> PISPIETVPVKLKPGMDGPKVKQWPLTEEKIKALVEICTEMEKEGKISKIGPENPYNTPVFAIKKKDSTKWRKLVDFRELNKRTQDFWEVQLGIPHPAGIKKKKSVTVLDVGDAYFSVPLDEDFRKYTAFTIPSINNETPGIRYQYNVLPQGWKGSPAIFQSSMTKILEPFRKQNPDIVIYQYMDDLYVGSDLEIGQHRTKIEELRQHLLRWGLTTPDKKHQKEPPFLWMGYELHPDKWTVQPIVLPEKDSWTVNDIQKLVGKLNWASQIYPGIKVRQLCKLLRGTKALTEVIPLTEEAELELAENREILKEPVHGVYYDPSKDLIAEIQKQGQGQWTYQIYQEPFKNLKTGKYARMRGAHTNDVKQLTEAVQKITTESIVIWGKTPKFKLPIQKETWETWWTEYWQATWIPEWEFVNTPPLVKLWYQLEKEPIVGAETFYVDGAANRETKLGKAGYVTNRGRQKVVTLTDTTNQKTELQAIYLALQDSGLEVNIVTDSQYALGIIQAQPDQSESELVNQIIEQLIKKEKVYLAWVPAHKGIGGNEQVDKLVSAGIRKVL;> PISPIETVPVKLKPGMDGPKVKQWPLTEEKIKALVEICTEMEKEGKISKIGPENPYNTPVFAIKKKDSTKWRKLVDFRELNKRTQDFWEVQLGIPHPAGIKKKKSVTVLDVGDAYFSVPLDEDFRKYTAFTIPSINNETPGIRYQYNVLPQGWKGSPAIFQSSMTKILEPFRKQNPDIVIYQYMDDLYVGSDLEI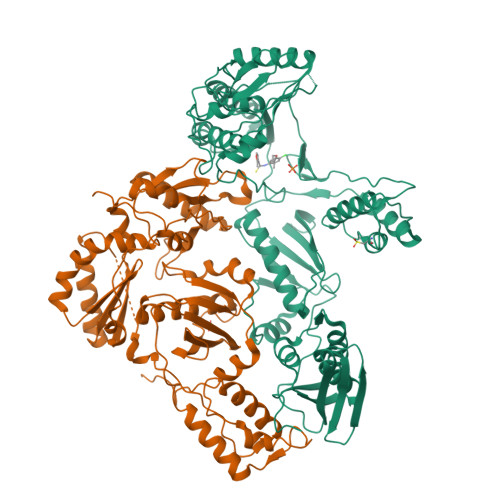GQHRTKIEELRQHLLRWGLTTPDKKHQKEPPFLWMGYELHPDKWTVQPIVLPEKDSWTVNDIQKLVGKLNWASQIYPGIKVRQLCKLLRGTKALTEVIPLTEEAELELAENREILKEPVHGVYYDPSKDLIAEIQKQGQGQWTYQIYQEPFKNLKTGKYARMRGAHTNDVKQLTEAVQKITTESIVIWGKTPKFKLPIQKETWETWWTEYWQATWIPEWEFVNTPPLVKLWYQLEKEPIVGAETF>[3x]MAFTGKFEMESEKNYDEFMKLLGISSDVIEKARNFKIVTEVQQDGQDFTWSQHYSGGHTMTNKFTVGKESNIQTMGG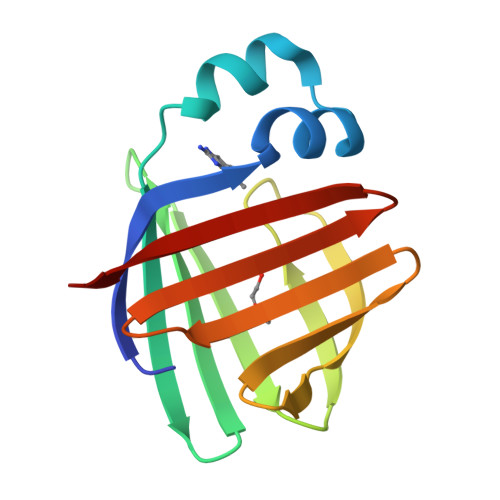KTFKATVQMEGGKLVVNFPNYHQTSEIVGDKLVEVSTIGGVTYERVSKRLA>[2x]DIYGDEITAVV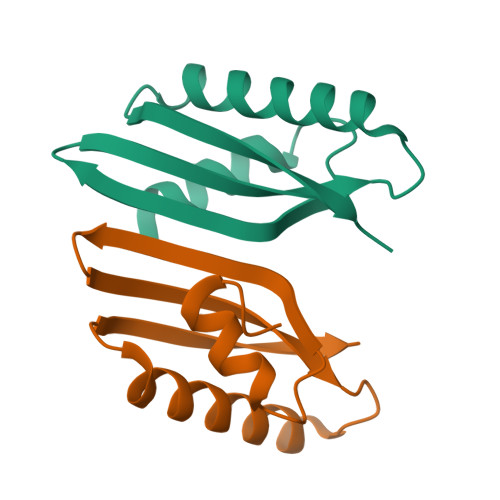SKIENVKGISQLKTRHIGQKIWAELNILVDPDSTIVQGETIASRVKKALTEQIRDIERVVVHFEPARK> AKMAFTLADRVTEEMLADKAALVVEVVEENYHDAPIVGIAVVNEHGRFFLRPETALADPQFVAWLGDETKKKSMFDSKRAAVALKWKGIELCGVSFDLLLAAYLLDPAQGVDDVAAAAKMKQYEAVRPDEAVYGKGAKRAVPDEPVLAEHLVRKAAAIWELERPFLDELRRNEQDRLLVELEQPLSSILAEMEFAGVKVDTKRLEQMGKELAEQLGTVEQRIYELAGQEFNINSPKQLGVILFEKLQLPVLKKTKTGYSTSADVLEKLAPYHEIVENILHYRQLGKLQSTYIEGLLKVVRPDTKKVHTIFNQALTQTGRLSSTEPNLQNIPIRLEEGRKIRQAFVPSESDWLIFAADYSQIELRVLAHIAEDDNLMEAFRRDLDIHTKTAMDIFQVSEDEVTPNMRRQAKAVNYGIVYGISDYGLAQNLNISRKEAAEFIERYFESFPGVKRYMENIVQEAKQKGYVTTLLHRRRYLPDITSRNFNVRSFAERMAMNTPIQGSAADIIKKAMIDLNARLKEERLQAHLLLQVHDELILEAPKEEMERLCRLVPEVMEQAVTLRVPLKVDYHYGSTWYD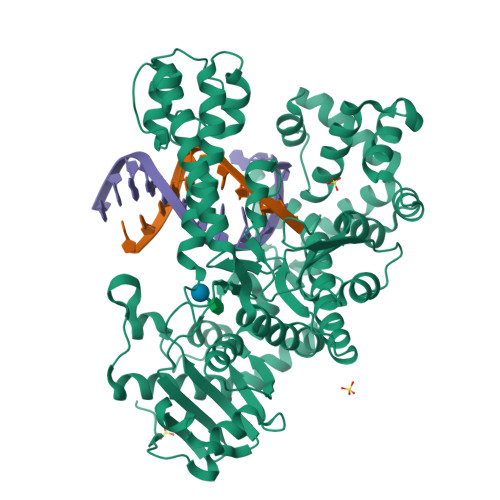AK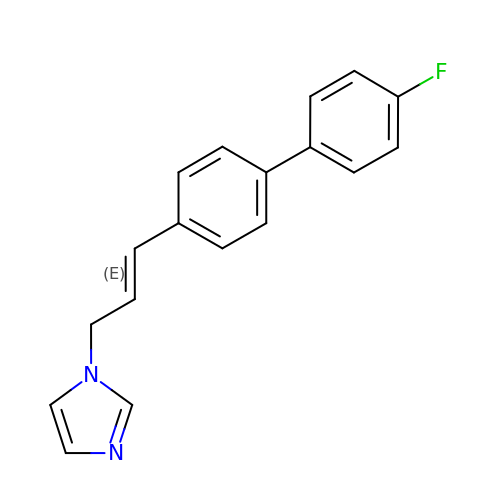1-[(~{E})-3-[4-(4-fluorophenyl)phenyl]prop-2-enyl]imidazole | C18 H15 F N2 | RYROXALRVYKQQD-OWOJBTEDSA-N> GSHMKNSVSVDLPGSMKVLVSKSSNADGKYDLIATVDALELSGTSDKNNGSGVLEGVKADASKVKLTISD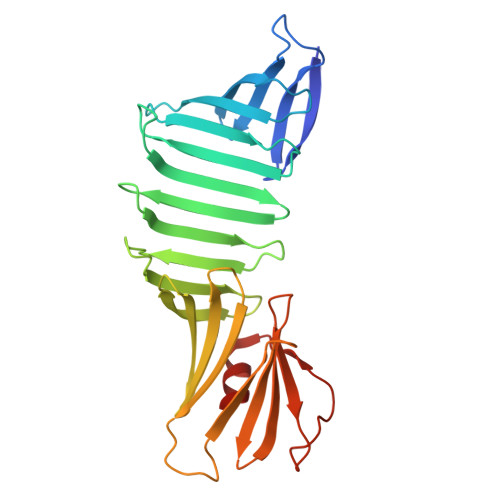DLGQTTLEVFKSDGSTLVSKKVTSNGSSTEEKIIDGIIIEKIITRADGTRLEYTGIKSDGSGKAKEVLKGYVLEGTLTAEKTTLVVKEGTVTLSKNISKSGEVSVELNDTDSSAATKKTAAWNSGTSTLTITVNSKKTKDLVFTSSNTITVQQYDSNGTSLEGSAVEITKLDEIKNALK>[5x]MNESVKEIPDVLKSQCGFNCLTDISHSSFNEFRQQVSEHLSWSETHDLYHDAQQAQKDNRLYEARILKRANPQLQNAVHLAILAPNAELIGYNNQFSGRASQYVAPGTVSSMFSPAAYLTELYREARNLHASDSVYYLDTRRPDLKSMALSQQNMDIELSTLSLSNELLLESIKTESKLENYTKVMEMLSTFRPSGATPYHDAYENVREVIQLQDPGLEQLNASPAIAGLMHQASLLGINASISPELFNILTEEITEGNAEELYKKNFGNIEPASLAMPEYLKRYYNLSDEELSQFIGKASNFGQQEYSNNQLITPVVNSSDGTVKVYRITREYTTNAYQMDVELFPFGGENYRLDYKFKNFYNASYLSIKLNDKRELVRTEGAPQVNIEYSANITLNTADISQPFEIGLTRVLPSGSWAYAAAKFTVEEYNQYSFLLKLNKAIRLSRATELSPTILEGIVRSVNLQLDINTDVLGKVFLTKYYMQRYAIHAETALILCNAPISQRSYDNQPSQFDRLFNTPLLNGQYFSTGDEEIDLNSGSTGDWRKTILKRAFNIDDVSLFRLLKITDHDNKDGKIKNNLKNLSNLYIGKLLADIHQLTIDELDLLLIAVGEGKTNLSAISDKQLATLIRKLNTITSWLHTQKWSVFQLFIMTSTSYNKTLTPEIKNLLDTVYHGLQGFDKDKADLLHVMAPYIAATLQLSSENVAHSVLLWADKLQPGDGAMTAEKFWDWLNTKYTPGSSEAVETQEHIVQYCQALAQLEMVYHSTGINENAFRLFVTKPEMFGAATGAAPAHDALSLIMLTRFADWVNALGEKASSVLAAFEANSLTAEQLADAMNLDANLLLQASIQAQNHQHLPPVTPENAFSCWTSINTILQWVNVAQQLNVAPQGVSALVGLDYIQSMKETPTYAQWENAAGVLTAGLNSQQANTLHAFLDESRSAALSTYYIRQVAKAAAAIKSRDDLYQYLLIDNQVSAAIKTTRIAEAIASIQLYVNRALENVEENANSGVISRQFFIDWDKYNKRYSTWAGVSQLVYYPENYIDPTMRIGQTKMMDALLQSVSQSQLNADTVEDAFMSYLTSFEQVANLKVISAYHDNINNDQGLTYFIGLSETDAGEYYWRSVDHSKFNDGKFAANAWSEWHKIDCPINPYKSTIRPVIYKSRLYLLWLEQKEITKQTGNSKDGYQTETDYRYELKLAHIRYDGTWNTPITFDVNKKISELKLEKNRAPGLYCAGYQGEDTLLVMFYNQQDTLDSYKNASMQGLYIFADMASKDMTPEQSNVYRDNSYQQFDTNNVRRVNNRYAEDYEIPSSVSSRKDYGWGDYYLSMVYNGDIPTINYKAASSDLKIYISPKLRIIHNGYEGQKRNQCNLMNKYGKLGDKFIVYTSLGVNPNNSSNKLMFYPVYQYSGNTSGLNQGRLLFHRDTTYPSKVEAWIPGAKRSLTNQNAAIGDDYATDSLNKPDDLKQYIFMTDSKGTATDVSGPVEINTAISPAKVQIIVKAGGKEQTFTADKDVSIQPSPSFDEMNYQFNALEIDGSGLNFINNSASIDVTFTAFAEDGRKLGYESFSIPVTLKVSTDNALTLHHNENGAQYMQWQSYRTRLNTLFARQLVARATTGIDTILSMETQNIQEPQLGKGFYATFVIPPYNLSTHGDERWFKLYIKHVVDNNSHIIYSGQLTDTNINITLFIPLDDVPLNQDYHAKVYMTFKKSPSDGTWWGPHFVRDDKGIVTINPKSILTHFESVNVLNNISSEPMDFSGANSLYFWELFYYTPMLVAQRLLHEQNFDEANRWLKYVWSPSGYIVHGQIQNYQWNVRPLLEDTSWNSDPLDSVDPDAVAQHDPMHYKVSTFMRTLDLLIARGDHAYRQLERDTLNEAKMWYMQALHLLGDKPYLPLSTTWSDPRLDRAADITTQNAHDSAIVALRQNIPTPAPLSLRSANTLTDLFLPQINEVMMNYWQTLAQRVYNLRHNLSIDGQPLYLPIYATPADPKALLSAAVATSQGGGKLPESFMSLWRFPHMLENARGMVSQLTQFGSTLQNIIERQDAEALNALLQNQAAELILTNLSIQDKTIEELDAEKTVLEKSKAGAQSRFDSYGKLYDENINAGENQAMTLRASAAGLTTAVQASRLAGAAADLVPNIFGFAGGGSRWGAIAEATGYVMEFSANVMNTEADKISQSETYRRRRQEWEIQRNNAEAELKQIDAQLKSLAVRREAAVLQKTSLKTQQEQTQSQLAFLQRKFSNQALYNWLRGRLAAIYFQFYDLAVARCLMAEQAYRWELNDDSARFIKPGAWQGTYAGLLAGETLMLSLA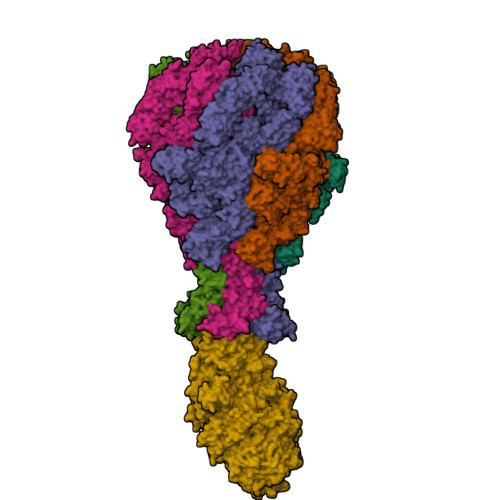QMEDAHLKRDKRALEVERTVSLAEVYAGLPKDNGPFSLAQEIDKLVSQGSGSAGSGNNNLAFGAGTDTKTSLQASVSFADLKIREDYPASLGKIRRIKQISVTLPALLGPYQDVQAILSYGDKAGLANGCEALAVSHGMNDSGQFQLDFNDGKFLPFEGIAIDQGTLTLSFPNASMPEKGKQATMLKTLNDIILHIRYTIK;> MQNSQDFSITELSLPKGGGAITGMGEALTPTGPDGMAALSLPLPISAGRGYAPAFTLNYNSGAGNSPFGLGWDCNVMTIRRRTHFGVPHYDETDTFLGPEGEVLVVADQPRDESTLQGINLGATFTVTGYRSRLESHFSRLEYWQPKTTGKTDFWLIYSPDGQVHLLGKSPQARISNPSQTTQTAQWLLEASVSSRGEQIYYQYRAEDDTGCEADEITHHLQATAQRYLHIVYYGNRTASETLPGLDGSAPSQADWLFYLVFDYGERSNNLKTPPAFSTTGSWLCRQDRFSRYEYGFEIRTRRLCRQVLMYHHLQALDSKITEHNGPTLVSRLILNYDESAIASTLVFVRRVGHEQDGNVVTLPPLELAYQDFSPRHHAHWQPMDVLANFNAIQRWQLVDLKGEGLPGLLYQDKGAWWYRSAQRLGEIGSDAVTWEKMQPLSVIPSLQSNASLVDINGDGQLDWVITGPGLRGYHSQRPDGSWTRFTPLNALPVEYTHPRAQLADLMGAGLSDLVLIGPKSVRLYANTRDGFAKGKDVVQSGDITLPVPGADPRKLVAFSDVLGSGQAHLVEVSATKVTCWPNLGRGRFGQPITLPGFSQPATEFNPAQVYLADLDGSGPTDLIYVHTNRLDIFLNKSGNGFAEPVTLRFPEGLRFDHTCQLQMADVQGLGVASLILSVPHMSPHHWRCDLTNMKPWLLNEMNNNMGVHHTLRYRSSSQFWLDEKAAALTTGQTPVCYLPFPIHTLWQTETEDEISGNKLVTTLRYARGAWDGREREFRGFGYVEQTDSHQLAQGNAPERTPPALTKNWYATGLPVIDNALSTEYWRDDQAFAGFSPRFTTWQDNKDVPLTPEDDNSRYWFNRALKGQLLRSELYGLDDSTNKHVPYTVTEFRSQVRRLQHTDSRYPVLWSSVVESRNYHYERIASDPQCSQNITLSSDRFGQPLKQLSVQYPRRQQPAINLYPDTLPDKLLANSYDDQQRQLRLTYQQSSWHHLTNNTVRVLGLPDSTRSDIFTYGAENVPAGGLNLELLSDKNSLIADDKPREYLGQQKTAYTDGQNTTPLQTPTRQALIAFTETTVFNQSTLSAFNGSIPSDKLSTTLEQAGYQQTNYLFPRTGEDKVWVAHHGYTDYGTAAQFWRPQKQSNTQLTGKITLIWDANYCVVVQTRDAAGLTTSAKYDWRFLTPVQLTDINDNQHLITLDALGRPITLRFWGTENGKMTGYSSPEKASFSPPSDVNAAIELKKPLPVAQCQVYAPESWMPVLSQKTFNRLAEQDWQKLYNARIITEDGRICTLAYRRWVQSQKAIPQLISLLNNGPRLPPHSLTLTTDRYDHDPEQQIRQQVVFSDGFGRLLQAAARHEAGMARQRNEDGSLIINVQHTENRWAVTGRTEYDNKGQPIRTYQPYFLNDWRYVSNDSARQEKEAYADTHVYDPIGREIKVITAKGWFRRTLFTPWFTVNEDENDTAAEVKKVKMMKNIDPKLYQKTPTVSVYDNRGLIIRNIDFHRTTANGDPDTRITRHQYDIHGHLNQSIDPRLYEAKQTNNTIKPNFLWQYDLTGNPLCTESIDAGRTVTLNDIEGRPLLTVTATGVIQTRQYETSSLPGRLLSVAEQTPEEKTSRITERLIWAGNTEAEKDHNLAGQCVRHYDTAGVTRLESLSLTGTVLSQSSQLLIDTQEANWTGDNETVWQNMLADDIYTTLSTFDATGALLTQTDAKGNIQRLAYDVAGQLNGSWLTLKGQTEQVIIKSLTYSAAGQKLREEHGNDVITEYSYEPETQRLIGIKTRRPSDTKVLQDLRYEYDPVGNVISIRNDAEATRFWHNQKVMPENTYTYDSLYQLISATGREMANIGQQSHQFPSPALPSDNNTYTNYTRTYTYDRGGNLTKIQHSSPATQNNYTTNITVSNRSNRAVLSTLTEDPAQVDALFDAGGHQNTLISGQNLNWNTRGELQQVTLVKRDKGANDDREWYRYSGDGRRMLKINEQQASNNAQTQRVTYLPNLELRLTQNSTATTEDLQVITVGEAGRAQVRVLHWESGKPEDIDNNQLRYSYDNLIGSSQLELDSEGQIISEEEYYPYGGTALWAARNQTEASYKTIRYSGKERDATGLYYYGYRYYQPWIGRWLSSAPAGTIDGLNLYRMVRNNPVTLLDPDGLMPTIAERIAALKKNKVTDSAPSPANATNVAINIRPPVAPKPSLPKASTSSQPTTHPIGAANIKPTTSGSSIVAPLSPVGNKSTSEISLPESAQSSSSSTTSTNLQKKSFTLYRADNRSFEEMQSKFPEGFKAWTPLDTKMARQFASIFIGQKDTSNLPKETVKNISTWGAKPKLKDLSNYIKYTKDKSTVWVSTAINTEAGGQSSGAPLHKIDMDLYEFAIDGQKLNPLPEGRTKNMVPSLLLDTPQIETSSIIALNHGPVNDAEISFLTTIPLKNVKPHKR>MGSDKIHHHHHHVINLKELKILHTSDWHLGVTSWTSSRPVDRREELKKALDKVVEEAEKREVDLILLTGDLLHSRNNPSVVALHDLLDYLKRMMRTAPVVVLPGNHDWKGLKLFGN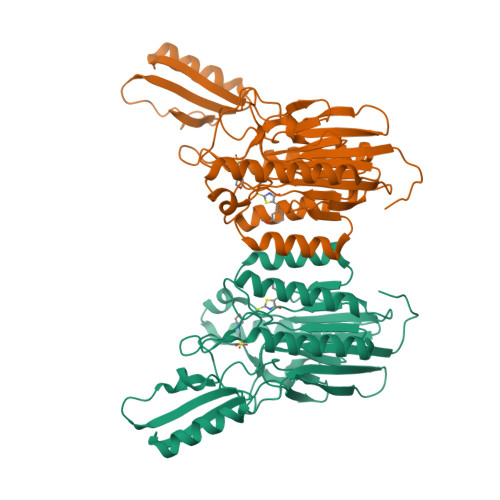FVTSISSDITFVMSFEPVDVEAKRGQKVRILPFPYPDESEALRKNEGDFRFFLESRLNKLYEEALKKEDFAIFMGHFTVEGLAGYAGIEQGREIIINRALIPSVVDYAALGHIHSFREIQKQPLTIYPGSLIRIDFGEEADEKGAVFVELKRGEPPRYERIDASPLPLKTLYYKKIDTSALKSIRDFCRNFPGYVRVVYEEDSGILPDLMGEIDNLVKIE[2x]>EGDIHMHHHHHHSSGLEVLFQGPGSISGSRTLEQSVGEWLESIGLQQYESKLLLNGFDDVRFLGSNVMEEQDLREIGISDPQHRRKLLQAARSLPKVKPSGSSGENLYFQSGSSGPEYPLFVTVGDW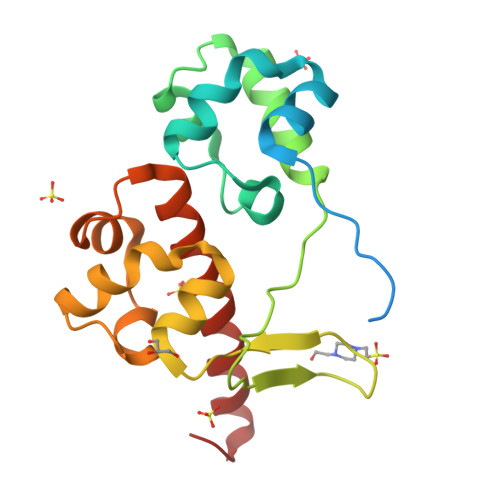LDSIKMGQYKSNFMAAGFTTFDLISRMSIDDIRRIGVILIGHQRRIVSSIQTLRLHMMHIQEKGFHV[2x]>[2x]SA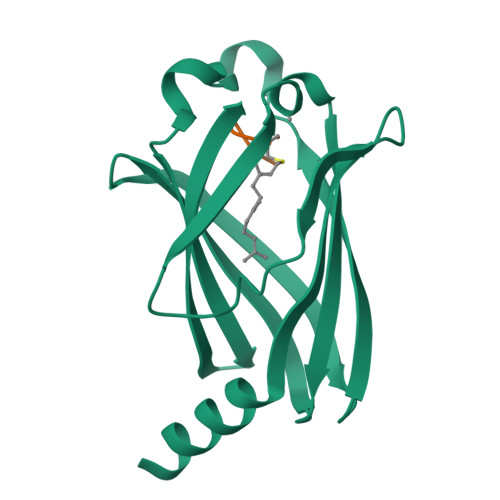KDERAREILRGFKLNWMNLRDAETGKILWQGTEDLSVPGVEHEARVPKKILKCKAVSRELNFSSTEQMEKFRLEQKVYFKGQCLEEWFFEFGFVIPNSTNTWQSLIEAAPESQMMPASVLTGNVIIETKFFDDDLLVSTSRVRLFYV;>[2x]SSTIC>[8x]MGSHHHHHHGRSAAGTMANLDKMLNTTVTEVRQFLQVDRVCVFQFEEDYSGVVVVEAVDDRWIS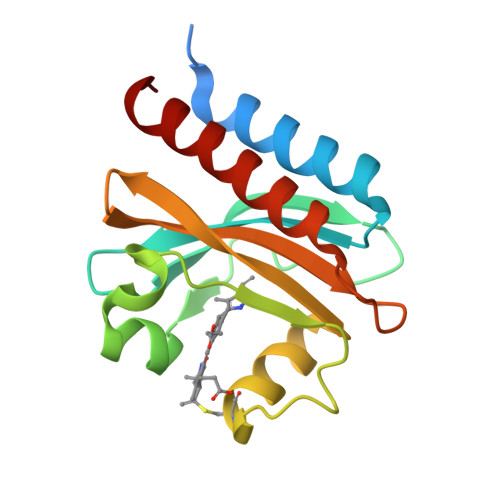ILKTQVRDRYFMETRGEEYSHGRYQAIADIYTANLTECYRDLLTQFQVRAILAVPILQGKKLWGLLVAHQLAAPRQWQTWEIDFLKQQAVVVGIAIQQS> MANDHINLKVAGQDGSVVQFKIKRHTPLS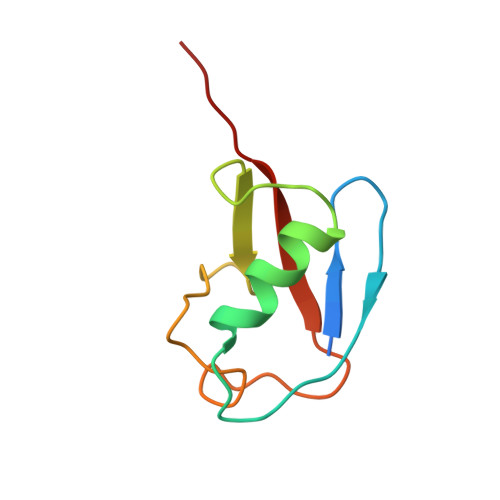KLMKAYCERQGLSMRQIRFRFDGQPINETDTPAQLEMEDEDTIDVFQQQTGG>[2x]GSNEKIRSQSVLNTLETFFIKENHYDMQREESSIVNACLRYLGYSKSMCHEKMPIFMDIAFIEYCFNLSLD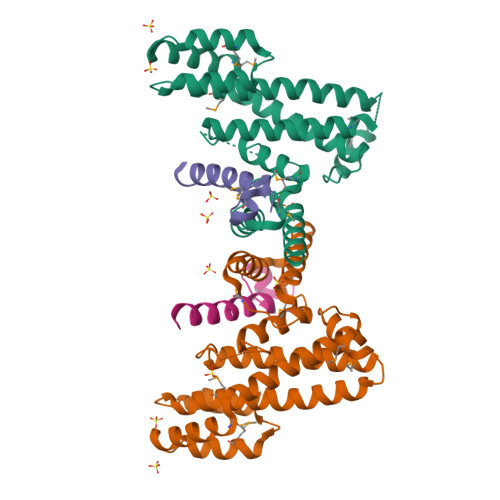PSSFQNLPITQTQPDSQQILWEYSLISNALERLENIELERQNCMREDGLVKYTNELLLNKETLNNEALKLYSCAKAGICRWMAFHFLEQEPIDHINFTKFLQDWGSHNEKEMEALQRLSKHKIRKRLIYVSQHKKKMPWSKFNSVLSRYIQCTKLQLEVFCDYDFKQREIVKMLTSNIN;>[2x]EACEMCRLGLPHGSFFELLRDWKKIEEFRNKS> MNLPTAQEVQGLMARFIELVDVGDIEAIVQMYADDATIESPFGQPPIHGRE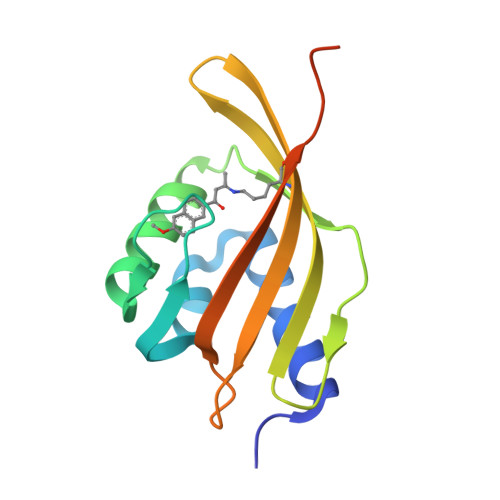QIAAHYRKWLGGGKLRVYLTGPVRANHNGCGTMLLRKEWVWNGQPCATDVILVMRFDEQGRIQTEQRYWSEVNLCVREPQGSLEHHHHHH>[2x]HHHHHHSSGENLYFQGHMDDYSTRSNDNRIKLVPIAPSRGMIFDRNGTPLALNRTIYQLELMPEKIENLSATLNALRPIVDLTDDDIANFEKERKRSRRFTSIAVKTPLTEVQVARFAVNQFRFPGIEVKGYQRRFYPYGSALTHVIGYVSKINDKDVERLDKEGILPNYAATHDIGKLGIERYYESTLHGKTGYEEVEVNNRGRVIRQLHEQPPQAGKDIYLTLDLSLQIYIEKLLSGSRAAVVVTDPRTGGILALVSNPSYDPNLFVDGISNKDYQGLLNDTNRPLINRATQGVYPPASTVKPYIAVSALSAG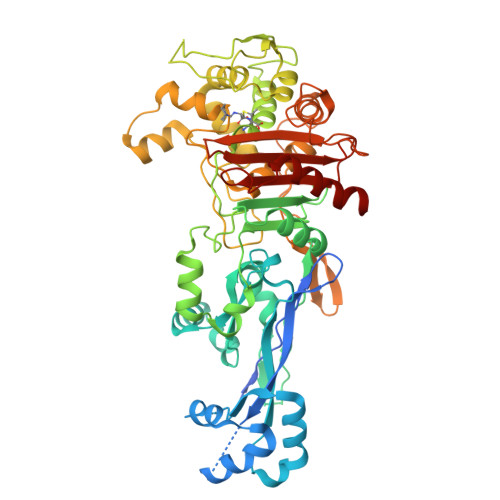VITKNTSLFDPGWWQLPGSEKRYRDWKKWGHGRLNVTKALEESADTFFYQVAYDMGIDRLSSWMSKFGYGEYTGIDLSEERAGLMPTREWKQKRHKKPWYQGDTIPVGIGQGYWTATPIQMAKSLMTLINDGTVKTPHLLQSTRIDGVLVPYKQEDSTQIGSINSGYWEIAKDGMYGVANRPNGTGRKFFEGTPYKAAAKSGTAQVYSYETYNASKVAEHLRDHKLMVAFAPYENPTVSVAIILENGGAGPAVGTITRQILDHILLGD>[6x]LYHNSQPTSSKPNLLVLPVQEDASTGLHWANIHKRTPLMQVPLLLDLNGKHLWVTCSQHYSSSTYQAPFCHSTQCSRANTHQCFTCTDSTTTRPGCHNNTCGLLSSNPVTQESGLGELAQDVLAIHSTHGSKLGPMVKVPQFLFSCAP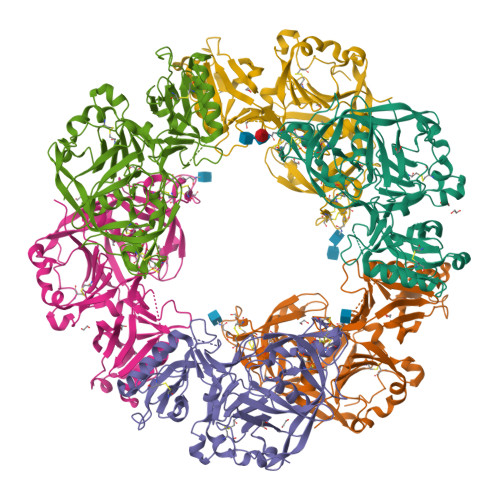SFLAQKGLPNNVQGALGLGQAPISLQNQLFSHFGLKRQFSVCLSRYSTSNGAILFGDINDPNNNNYIHNSLDVLHDLVYTPLTISKQGEYFIQVNAIRVNKHLVIPTKNPFISPSSTSYHGSGEIGGALITTTHPYTVLSHSIFEVFTQVFANNMPKQAQVKAVGPFGLCYDSRKISGGAPSVDLILDKNDAVWRISSENFMVQAQDGVSCLGFVDGGVHARAGIALGAHHLEENLVVFDLERSRVGFNSNSLKSYGKTCSNLFDLNNP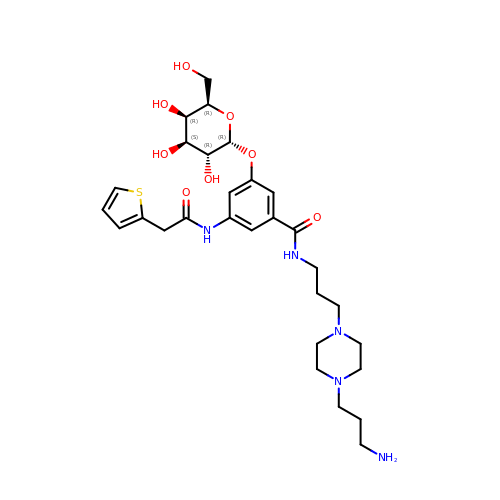N-{3-[4-(3-AMINO-PROPYL)-PIPERAZIN-1-YL]-PROPYL}-3-(2-THIOPHEN-2-YL-ACETYLAMINO)-5-(3,4,5-TRIHYDROXY-6-HYDROXYMETHYL-TETRAHYDRO-PYRAN-2-YLOXY)-BENZAMIDE | C29 H43 N5 O8 S | ZIXIINLBMSXOQV-ADWZMSLQSA-N> GPLSLSVDAFKILEDPKWEFPRKNLVLGKTLGEGEFGKVVKATAFHLKGRAGYTTVAVKMLKENASPSELRDLLSEFNVLKQVNHPHVIKLYGACSQDGPLLLIVEYAKYGSLRGFLRESRKVGPGYLG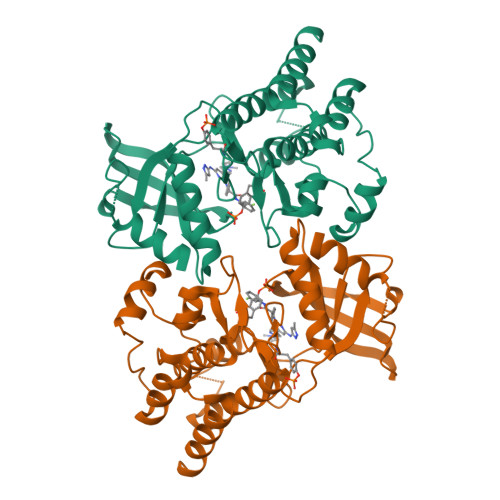SGGSRNSSSLDHPDERALTMGDLISFAWQISQGMQYLAEMKLVHRDLAARNILVAEGRKMKISDFGLSRDVYEEDSYVKRSQGRIPVKWMAIESLFDHIYTTQSDVWSFGVLLWEIVTLGGNPYPGIPPERLFNLLKTGHRMERPDNCSEEMYRLMLQCWKQEPDKRPVFADISKDLEKMMVKRR>MAEKPKLHYFNARGRMESTRALLAAAGVEFEEKFIKSAEDLDKLRNDGYLMFQQVPMVEIDGMKLVQTRAILNYIASKYNLYGKDIKERALIDMYIEGIADLGEMILLLPVCPPEEKDAKLALIKEKIKNRYFPAFEKVLKSHGQDYLVGNKLSRADIHLVELLYYVEELDSSLISS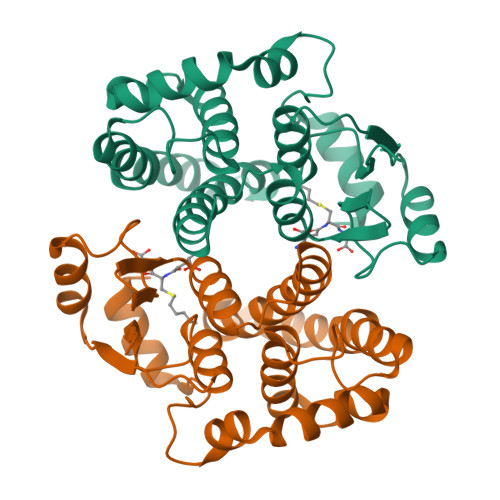FPLLKALKTRISNLPTVKKFLQPGSPRKPPMDEKSLEEARKIFRF[2x]> MEIDPKDLTFLKELGTGQFGVVKYGKWRGQYDVAIRMIREGSMSEDEFIEEAKVMMNLSHEKLVQLYGVCTKQRPIFIITEYMANGCLLNYLREMRHRFQTQQLLEMCKDVCEAMEYLESKQFLHRDLAARNCLVNDQGVV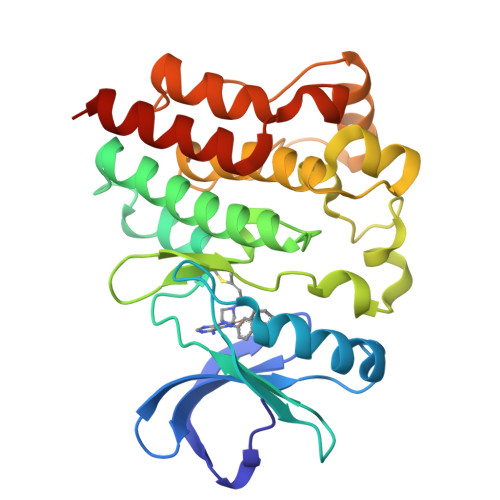KVSDFGMTRYVLDDEYTSSTGSKFPVKWASPEVLMYSKFSSKSDIWAFGVLMWEIYSLGKMPYERFTNSETAEHIAQGLRLPRPHLASERVYTIMYSCWHEKADERPSFKILLSNILDVMDEESHHHHHH>MRSVEQQLSIVTEAAVAPEPVRIAIAEALGLMCAEEVQASRALPGFAQAAIDGYAVRAVDVGGEKSLSQQLPVAPPEKSLPVVGEVAAGSQQPLRLQPKQAVMVHTGAPLPMLADAVLPMAWSDRGRKRVTAQRPVRSGEFVRKEGDDIQPGDIAVSAGAVLGPAQIGLLAAVGRSKVLVYPRPRMSVISVGAELVDIDRQPGLGQVYDVNSYSLAAAGREAGADVYRYGIAAGEPRRIKEIIESQMLRSEIIVITGAVGGAGSAGVRQVLNELGDIDTERVAMHPGSVQGFGLLGENKIPCFLLPSNPVASLVIFETFVRPVVRMSLGKSNAARRVVRARALNHVVSVAGRKGFIRSRLMRDAETQDYLVEALGGATGAPSHLLAGLSEANGMIRIPEDVTEIRPGDVVDVIFLAQGR[2x]

In this work we have identified Glp, a gephyrin-like repurposed molybdotransferase MoeA enzyme, and its membrane receptor, GlpR, as components of the corynebacterial divisome. Our studies show that Glp and GlpR form a tight complex that is part of the early divisome, where Glp and GlpR directly bind FtsZ and Wag31, respectively, placing the Glp–GlpR complex at the centre of the divisome–elongasome transition.

We crystallized Glp alone and in complex with the 10-residue peptide FtsZCTD. The apo-structure was solved at 2.1 Å resolution and the structure of the complex was solved at 2.7 Å resolution. The structure of Glp is consistent with its annotation as MoeA, the enzyme involved in the synthesis of the molybdenum co-factor (Moco), which is present in all forms of life and is used by molybdoenzymes to mediate essential cellular functions such as energy generation and detoxification reactions, and to support virulence in pathogenic bacteria. However, a pronounced hinge motion around the segments connecting structural domains I and III leads to an open form of the Glp homodimer compared with the closed form of E. coli MoeA. This conformational change, also seen in the absence of ligand, generates the FtsZ-binding site within the central Glp dimer interface, far from the putative Mo-active site. In the phylogeny of these homologues, we identified a monophyletic clade that contains Cglu Glp and whose sequences are distinguished by two conserved proline-rich (pro-rich) regions. These regions correspond to the linkers connecting structural domains I and III, which differ between Glp and E. coli MoeA and are responsible for the hinge motion that generates the FtsZ-binding site in the former.> MTQWKNALSEGQLQQALELLIEAIKASPKDASLRSSFIELLCIDGDFERADEQLMQSIKLFPEYLPGASQLRHLVKAAQARKDFAQGAATAKVLGENEELTKSLVSF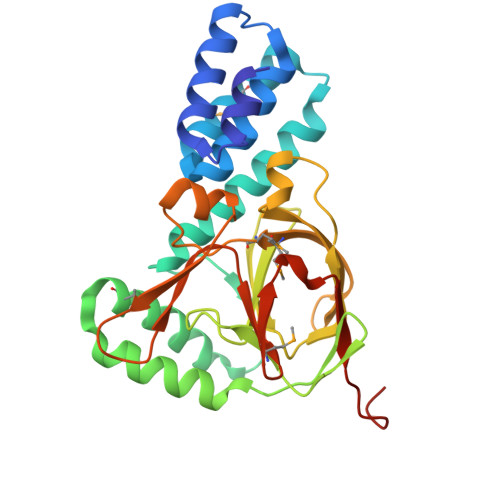NLSMVSQDYEQVSELALQIEELRQEKGFLANDTSFSDVRDIDDRLGGYIELFSTAGNYFLVPIASINTLEIKSATSLLESVWRPVEFDIDGLGEGEGHMPMTYVDSESDAQKLGRETDWKQIADKEVYLGLGLKCWLVGEMALPISDLQNLQVIKELALEHHHHHH>ARPCIPKSFGYSSVVCVCNATYCDSFDPPTFPALGTFSRYESTRSGRRMELSMGPIQANHTGTGLLLTLQPEQKFQKVKGFGGAMTDAAALNILALSPPAQNLLLKSYFSEEGIGYNIIRVPMASCDFSIRTYTYADTPDDFQLHNFSLPEEDTKLKIPLIHRALQLAQRPVSLLASPWTSPTWLKTNGAVNGKGSLKGQPGDIYHQTWARYFVKFLDAYAEHKLQFWAVTAENEPSAGLLSGYPFQCLGFTPEHQRDFIARDLGPTLANSTHHNVRLLMLDDQRLLLPHWAKVVLTDPEAAKYVHGIAVHWYLDFLAPAKATLGETHRLFPNTMLFASEACVGSKFWEQSVRLGSWDRGMQYSHSIITSLLYHVVGWTDWNLALNPEGGPNWVRNFVDSPIIVDITKDTFYKQPMFYHLGHFSKFIPEGSQRVGLVASQ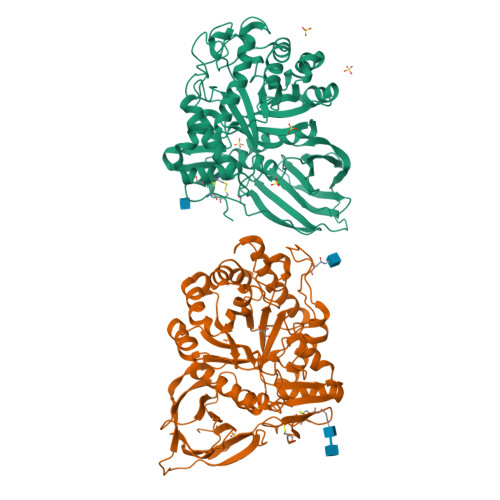KNDLDAVALMHPDGSAVVVVLNRSSKDVPLTIKDPAVGFLETISPGYSIHTYLWRRQ[2x]>[2x]GSLEMAEPQAESEPAAGGARGGGGDWPAGLTTYRSIQVGPGAAARWDLCIDQAVVFIEDAIQYRSINHRVDASSMWLYRRYYSNVCQRTLSFTIFLILFLAFIETPSSLTSTADVRYRAAPWEPPCGLTESVEVLCLLVFAADLSVKGYLFGWAHFQKNLWLLGYLVVLVVSLVDWTVSLSLVCHEPLRIRRLLRPFFLLQNSSMMKKTLKCIRWSLPEMASVGLLLAIHLCLFTMFGMLLFAGGKQDDGQDRERLTYFQNLPESLTSLLVLLTTANNPDVMIPAYSKNRAYAIFFIVFTVIGSLFLMNLLTAIIYSQFRGYLMKSLQTSLFRRRLGTRAAFEVLSSMVGEGGAFPQAVGVKPQNLLQVLQKVQLDSSHKQAMMEKVRSYGSVLLSAEEFQKLFNELDRSVVKEHPPRPEYQSPFLQSAQFLFGHYYFDYLGNLIALANLVSICVFLVLDADVLPAERDDFILGILNCVFIVYYLLE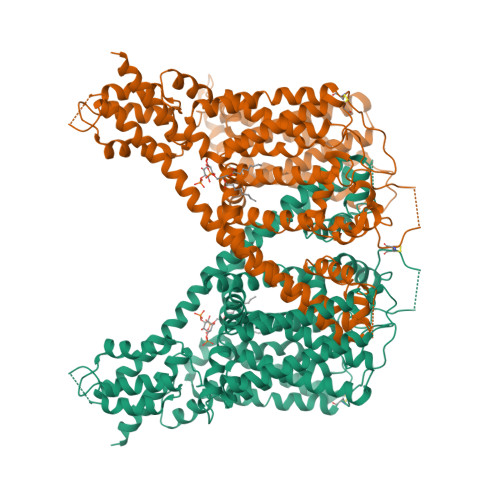MLLKVFALGLRGYLSYPSNVFDGLLTVVLLVLEISTLAVYRLPHPGWRPEMVGLLSLWDMTRMLNMLIVFRFLRIIPSMKPMAVVASTVLGLVQNMRAFGGILVVVYYVFAIIGINLFRGVIVALPGNSSLAPANGSAPCGSFEQLEYWANNFDDFAAALVTLWNLMVVNNWQVFLDAYRRYSGPWSKIYFVLWWLVSSVIWVNLFLALILENFLHKWDPRSHLQPLAGTPEATYQMTVELLFRDILEEPEEDELTERLSQHPHLWLCR> AAAADTTVTQFLQSFKENAENGALRKFYEVIMDNGGAVLDDINSLTEVTILAPSNEAWNSSNINNVLRDRNKMRQILNMHIIKDRLNVDKIRQKNANLIAQVPTVNNNTFLYFNVRGEGS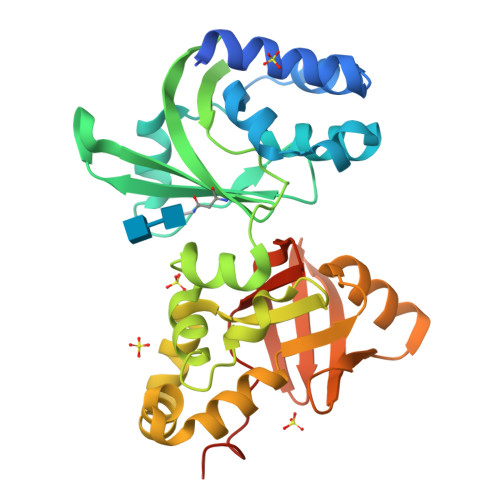DTVITVEGGGVNATVIQADVAQTNGYVHIIDHVLGVPYTTVLGKLESDPMMSDTYKMGKFSHFNDQLNNTQRRFTYFVPRDKGWQKTELDYPSAHKKLFMADFSYHSKSILERHLAISDKEYTMKDLVKFSQESGSVILPTFRDSLSIRVEEEAGRYVIIWNYKKINVYRPDVECTNGIIHVIDYPLLEEKDVVVAGGSAAAAA>MITILGAGKVGMATAVMLMMRGYDDLLLIARTPGKPQGEALDLAHAAAELGVDIRISGSNSYEDMRGSDIVLVTAGIGRKPGMTREQLLEANANTMADLAEKIKAYAKDAIVVITTNPVDAMTYVMYKKTGFPRERVIGFSGILDSARMAYYISQKLGVSFKSVNAIVLGMHGQKMFPVPRLSSVGGVPLEHLMSKEEIEEVVSETVNA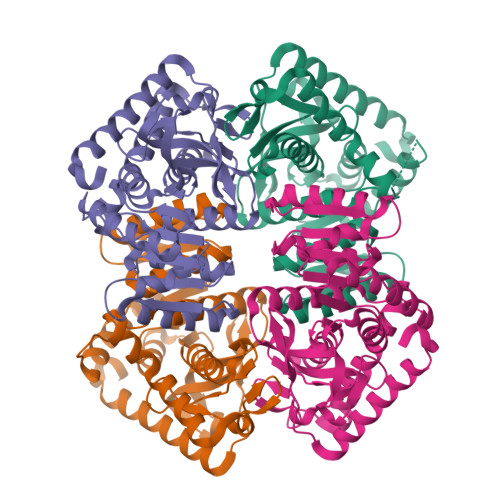GAKITELRGYSSNYGPAAGLVLTVEAIKRDSKRIYPYSLYLQGEYGYNDIVAEVPAVIGKSGIERIIELPLTEDEKRKFDEAVQAVKKLVETLPPQLRE[4x]ETX0462 (Bound form) | C10 H16 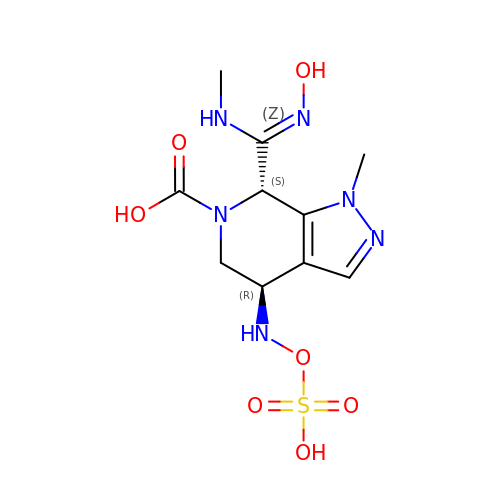N6 O7 S | TVYRNFNEBLNAMJ-XPUUQOCRSA-N>[2x]MADPGDRLGVLTTTRRVVEQAQAVWIDHDAVAQIAEAFAARQVTPPTWNRELHWSDGREALANYILVLDAVNFCFWGEPRWRIEYAGAVYDGYWALAASLKRALEQGVPLTDASYLAEITRDDVATIFAGEGEIPLLDERARIL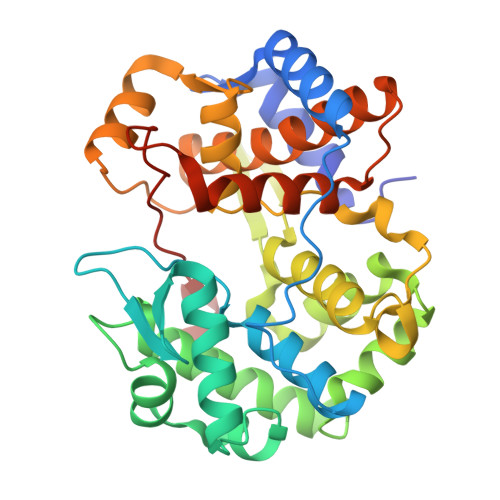RETGSVLAERFAGRFSDAIAAAGRSAVALVDIVTNAFPSFRDVATYRGEQVRFYKRAQILVSDLYGAFDGSDLGAFDDLGELTAFADYKVPQVLHHLGILRYAPALHDRLARREEIPAGSPEEVEIRAATIWGVEELRRALASRGHALDAYQVDWLLWDEGQRLPAGTLPYHRTRTIFYLEHHHHHH> IPEPKPGDLIEIFRPFYRHWAIYVGDGYVVHLAPPSEVAGAGAASVMSALTDKAIVKKELLYDVAGSDKYQVNNKHDDKYSPLPCSKIIQRAEELVGQEVLYKLTSENCEHFVNELRYGVAHHHHHH

The small GTPase RAS proteins operate as “molecular switches” that fluctuate between inactive and active states. These switches can be activated by the exchange of guanosine triphosphate (GTP) for guanosine diphosphate (GDP), which is promoted by guanine nucleotide exchange factors (GEFs). The H-REV107 gene is a known member of the class II tumor suppressor gene family that has been identified as a growth inhibitory RAS target capable of suppressing anchorage independent growth in vitro an in vivo. Here, we found direct interaction and inhibition between KRAS G12V and novel H-REV107 peptide.

Several studies have shown that H-REV107 is ubiquitously expressed in most normal tissues, however, expression is lost in human tumor cell lines and tumor samples. In contrast, induction of H-REV107 expression resulted in growth inhibition of RAS-transformed cells in vitro and in vivo. Characterizing the molecular details describing how H-REV107 binds KRAS G12V is essential to understanding the molecular mechanism through which H-REV107 inhibits oncogenic KRAS mutants. It is known that the H-REV107 protein family can inhibit the RAS signaling pathway, but the molecular mechanism responsible for this is unknown. We obtained the fraction crystal of the N-terminal domain (residues 1–125), but the electron density for residues 1–4 and 40–56 was poor. The crystal belonged to the orthorhombic P212121, with unit cell parameters a = 42.935 Å, b = 52.997 Å, c = 62.796 Å, and α = β = γ = 90 o. The structure of H-REV107 comprises four α-helices (α1–α4) and six β-strands (β1–β6). The H-REV107 peptide was synthesized in a water-soluble form and its fraction was designed from α1 to β5 (amino acids 65–74).4-[[(2~{R})-1-[4-(3-chlorophenyl)phenyl]-4-oxidanyl-4-oxidanylidene-butan-2-yl]amino]-4-oxidanylidene-butanoic acid | C20 H20 Cl N O5 | 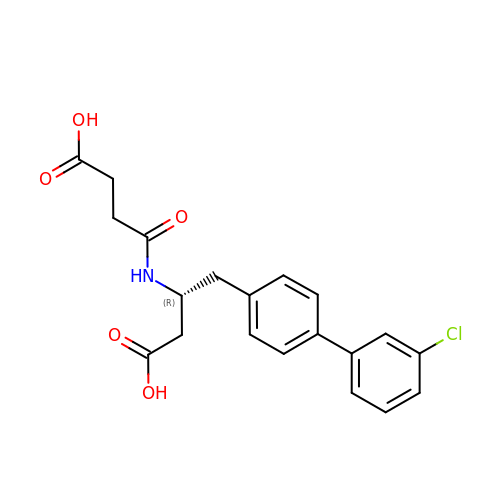ZBGYPMPWJWNWEA-QGZVFWFLSA-N>[7x]MHHHHHHGMASMTARPLSELVERGWAAALEPVADQVAHMGQFLRAEIAAGRRYLPAGSNVLRAFTFPFDNVRVLIVGQDPYPTPGHAVGLSFSVAPDVRPWPRSLANIFDEYTADLGYPLPSNGD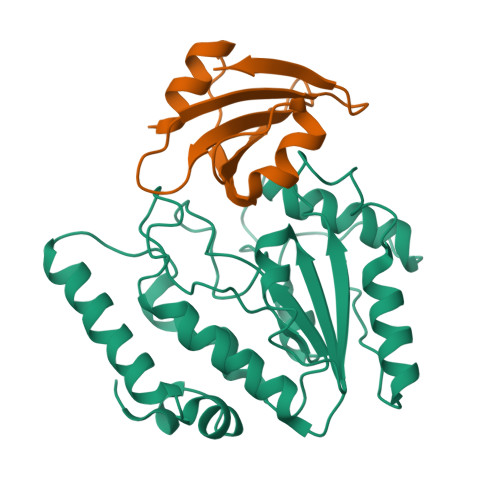LTPWAQRGVLLLNRVLTVRPSNPASHRGKGWEAVTECAIRALAARAAPLVAILWGRDASTLKPMLAAGNCVAIESPHPSPLSASRGFFGSRPFSRANELLVGMGAEPIDWRLP;>[7x]MTNLSDIIEKETGKQLVIQESILMLPEEVEEVIGNKPESDILVHTAYDESTDENVMLLTSDAPEYKPWALVIQDSNGENKIKML>MAHHHHHHMVIIPARFASTRLPGKPLQDINGKPMIVHVLERARESGADRIIVATDHEDVARAVEAAGGEVCMTRADHQSGTERLAEVVEKCAFSDDTI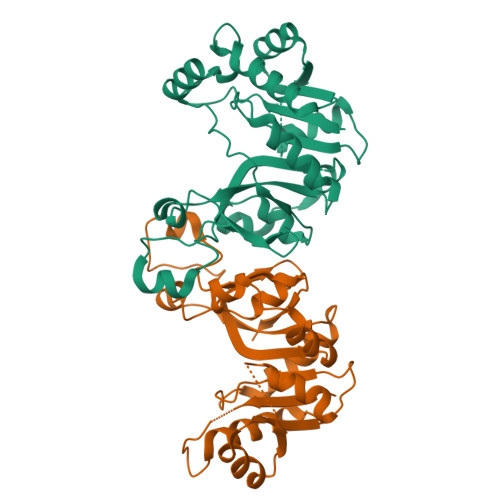IVNIQGDEPMIPPAIVRQVAENLAASSSGMATLAVPIHDAEEAFNPNAVKVVMDAKGYALYFSRATIPWDRDRFAQSRETIGDSLLRHIGIYGYRAGFIRRYVSWAPSPLEQIEMLEQLRVLWYGEKIHVAVAAEVPGTGVDTPEDLERVRAELR[2x]>[4x]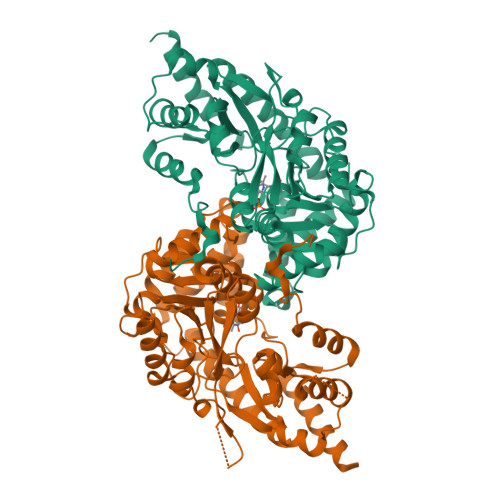MAKQLQARRLDGIDYNPWVEFVKLASEHDVVNLGQGFPDFPPPDFAVEAFQHAVSGDFMLNQYTKTFGYPPLTKILASFFGELLGQEIDPLRNVLVTVGGYGALFTAFQALVDEGDEVIIIEPFFDCYEPMTMMAGGRPVFVSLKPGPIQNGELGSSSNWQLDPMELAGKFTSRTKALVLNTPNNPLGKVFSREELELVASLCQQHDVVCITDEVYQWMVYDGHQHISIASLPGMWERTLTIGSAGKTFSATGWKVGWVLGPDHIMKHLRTVHQNSVFHCPTQSQAAVAESFEREQLLFRQPSSYFVQFPQAMQRCRDHMIRSLQSVGLKPIIPQGSYFLITDISDFKRKMPDLPGAVDEPYDRRFVKWMIKNKGLVAIPVSIFYSVPHQKHFDHYIRFCFVKDEATLQAMDEKLRKWKVELENLYFQGKGGRADPAFLYKVVRMNEDLGKPIPNPLLGLDSTRTGHHHHHH> HMSTGDFLTKGIELVQKAIDLDTATQYEEAY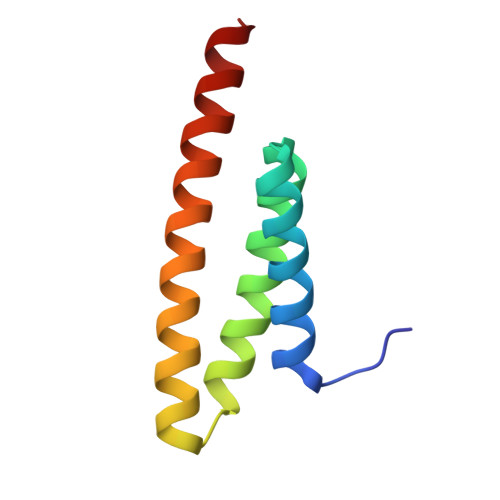TAYYNGLDYLMLALKYEKNPKSKDLIRAKFTEYLNRAEQLKKHLESEEANAA> MNYNLSKYPDDVSRLFKPRPPLSYKRPTDYPYAKRQTNPNITGVANLLSTSLKHYMEEFPEGSPNNHLQRYEDIKLSKIKNAQLLDRRLQNWNPNVDPHIKDTDPYRTIFIGRLPYDLDEIELQKYFVKFGEIEKIRIVKDKITQKSKGYAFIVFKDPISSKMAFKEIGVHRGIQIKDRICIVDIERGRTVKYFKPRRLGGGLGGRGYSNRDSRLPGRFASASTSNPAERNYAPRLPRRETSSSAYSADRYGSSTLDARYRGNRPLLSAATPTAAVTSVYKSRNSRTRESQPAPKEAPDY;> MPKFYCDYCDTYLTHDSPSVRKTHCSGRKHKENVKDYYRNKARDIINKHNHKRRHIGKRGRKERENSSQNETLKVTCLSNKEKRHIMHVKKMNQKELAQTSIDTLKLLYDGSPGYSKVFVDANRFDIGDLVKASKLPQRANEKSAHHSFKQTSRSRDETCESNPFPRLNNPKKLEPPKILSQWSNTIPKTSIFYSVDILQTTIKESKKRMHSDGIRKPSSANGYKRRRYGN;> MSALYFQNLPSRPANKENYTRLLLKHINPNNKYAINPSLPLPHNKLQISSQPLMLLDDQMGLLEVSISRSSKMTNQAFLTFVTQEEADRFLEKYTTTALKVQGRKVRMGKARTNSLLGLSIEMQKKKGNDETYNLDIKKVLKARKLKRKLRSDDICAKKFRLKRQIRRLKHKLRSRKVEEAEIDRIVKEFETRRLENMKSQQENLKQSQKPLKRAKVSNTMENPPNKVLLIQNLPSGTTEQLLSQILGNEALVEIRLVSVRNLAFVEYETVADATKIKNQLGSTYKLQNNDVTIGFAKGRRIPGLINPWKRRWKKNFIAVSAANRFKKISSSGALDYDIPTTASENLYFQ;> MDKYTALIHDENFSTLTLNVSRYPKSLAYWEKLLNYIVKASAPICKSTEPQLLKLIRCTYSSMLNEFPYLENYYIDFALLEYKLGNVSMSHKIFQRGLQAFNQRSLLLWTSYLKFCNNVISHQKQLFKKYETAEEYVGLHFFSGEFWDLYLEQISSRCTSSKKYWNVLRKILEIPLHSFSKFYALWLQRIDDIMDLKQLSQLTSKDELLKKLKIDINYSGRKGPYLQDAKKKLKKITKEMYMVVQYQVLEIYSIFESKIYINYYTSPETLVSSDEIETWIKYLDYTITLQTDSLTHLNFQRALLPLAHYDLVWIKYSKWLINSKNDLLGAKNVLLMGLKFSLKKTEIIKLLYSVICKLNEYVLLRNLLEKIESSYSDNVENVDDFEIFWDYLQFKTFCQNSLYSSRYSDSQSNGLLNKELFDKVWKRLSCKEKKSGQEILLNNLVQFYSKDTVEFVEKNIFQKIIEFGWEYYLQNGMFWNCYCRLIYFDTSRSYLDKRQYIVRKIWPQIDKKFAQSVLPSLTEFCESYFPEEMDTLEEMFTEEP;> MPDETNFTIEDIEPRPDALRGLDTQFLQDNTALVQAYRGLDWSDISSLTQMVDVIEQTVVKYGNPNDSIKLALETILWQILRKYPLLFGFWKRFATIEYQLFGLKKSIAVLATSVKWFPTSLELWCDYLNVLCVNNPNETDFIRNNFEIAKDLIGKQFLSHPFWDKFIEFEVGQKNWHNVQRIYEYIIEVPLHQYARFFTSYKKFLNEKNLKTTRNIDIVLRKTQTTVNEIWQFESKIKQPFFNLGQVLNDDLENWSRYLKFVTDPSKSLDKEFVMSVFDRCLIPCLYHENTWMMYIKWLTKKNISDEVVVDIYQKANTFLPLDFKTLRYDFLRFLKRKYRSNNTLFNNIFNETVSRYLKIWPNDILLMTEYLCMLKRHSFKNSLDQSPKEILEKQTSFTKILETSITNYINNQIDAKVHLQTLINDKNLSIVVVELIKTTWLVLKNNMQTRKYFNLYQKNILIKNSVPFWLTYYKFEKSNVNFTKLNKFIRELGVEIYLPTTVMNDILTDYKTFYLTHSNIVTYESSIIDSNTFDPILYPELKMSNPKYDPVLNTTANVDWHKKTEWKEAGHIGITTERPQISNSIIECNSGTLIQKPISLPNFRNLEKINQVKINDLYTEEFLKEGK;> MSYKQTTYYPSRGNLVRNDSSPYTNTISSETNNSSTSVLSLQGASNVSLGTTGNQLYMGDLDPTWDKNTVRQIWASLGEANINVRMMWNNTLNNGSRSSMGPKNNQGYCFVDFPSSTHAANALLKNGMLIPNFPNKKLKLNWATSSYSNSNNSLNNVKSGNNCSIFVGDLAPNVTESQLFELFINRYASTSHAKIVHDQVTGMSKGYGFVKFTNSDEQQLALSEMQGVFLNGRAIKVGPTSGQQQHVSGNNDYNRSSSSLNNENVDSRFLSKGQSFLSNGNNNMGFKRNHMSQFIYPVQQQPSLNHFTDPNNTTV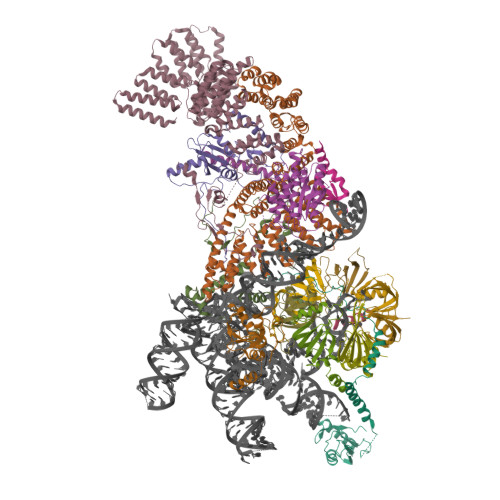FIGGLSSLVTEDELRAYFQPFGTIVYVKIPVGKCCGFVQYVDRLSAEAAIAGMQGFPIANSRVRLSWGRSAKQTALLQQAMLSNSLQVQQQQPGLQQPNYGYIPSSTCEAPVLPDNNVSSTMLPGCQILNYSNPYANANGLGSNNFSFYSNNNATNTQATSLLADTSSMDLSGTGGQQVIMQGSEAVVNSTNAMLNRLEQGSNGFMFA;> MRPRRRGLAYHHTKPKGQLSQGHYPTTSNDGQRRKVGNSEAFQSFDIWKNLDRIRSTKKNAGQFIKGSLLILPMRTEDKQQFDECMDELHKYISKDILRCYPQKEQKDEGMLFYIVLKDFNILDSCFVLSVLLAFQKRLWMAPSEKSYFRVPKNINLTGSFYLPKNIETGRGHIITSYRREQPSSSIVEVGFNVVPDFQQFQVKACHVSKFMNELSNFFSQVEFGKCEANVINYFKREYNRTYSQISLALYELPLIGDGLFDIKSYISKTRPIIETSKAQMIKHISEMKAYNEISGLQGDQFPRQQRPLSNSPSSNSISSSQTIEAGATSYQTQPQRHAVNKPSNVLNSSNRHSGPKTFEDGRYSEGNKPGFMTQDEIKQHCIGTIKASMDAVKKKSSYQILKTYVRCPRQNYIDIVYQNLNDLRSKTNCNIVVLNLNNLHESQMWLESLNTTNYTIFAQAPHPSTIRVISIGGVGEYIVKALELILNILEH;> MRDIVFVSPQLYLSSQEGWKSDSAKSGFIPILKNDLQRFQDSLKHIVDARNS;> MSTMSTPAAEQRKLVEQLMGRDFSFRHNRYSHQKRDLGLHDPKICKSYLVGECPYDLFQGTKQSLGKCPQMHLTKHKIQYEREVKQGKTFPEFEREYLAILSRFVNECNGQISVALQNLKHTAEERMKIQQVTEELDVLDVRIGLMGQEIDSLIRADEVSMGMLQSVKLQELISKRKEVAKRVRNITENVGQSAQQKLQVCEVCGAYLSRLDTDRRLADHFLGKIHLGYVKMREDYDRLMKNNRTTNASKTATTLPGRRFV;> MSKIQVAHSSRLANLIDYKLRVLTQDGRVYIGQLMAFDKHMNLVLNECIEERVPKTQLDKLRPRKDSKDGTTLNIKVEKRVLGLTILRGEQILSTVVEDKPLLSKKERLVRDKKEKKQAQKQTKLRKEKEKKPGKIAKPNTANAKHTSSNSREIAQPSSSRYNGGNDNIGANRSRFNNEAPPQTRKFQPPPGFKRK;> MKLVNFLKKLRNEQVTIELKNGTTVWGTLQSVSPQMNAILTDVKLTLPQPRLNKLNSNGIAMASLYLTGGQQPTASDNIASLQYINIRGNTIRQIILPDSLNLDSLLVDQKQLNSLRRSGQIANDPSKKRRRDFGAPANKRPRRGL;> MSSQIIDRPKHELSRAELEELEEFEFKHGPMSLINDAMVTRTPVIISLRNNHKIIARVKAFDRHCNMVLENVKELWTEKKGKNVINRERFISKLFLRGDSVIVVLKTPVE;> MTMNGIPVKLLNEAQGHIVSLELTTGATYRGKLVESEDSMNVQLRDVIATEPQGAVTHMDQIFVRGSQIKFIVVPDLLKNAPLFKKNSSRPMPPIRGPKRR;> MSNKVKTKAMVPPINCIFNFLQQQTPVTIWLFEQIGIRIKGKIVGFDEFMNVVIDEAVEIPVNSADGKEDVEKGTPLGKILLKGDNITLITSAD;> MSESSDISAMQPVNPKPFLKGLVNHRVGVKLKFNSTEYRGTLVSTDNYFNLQLNEAEEFVAGVSHGTLGEIFIRCNNVLYIRELPN;> MVSTPELKKYMDKKILLNINGSRKVAGILRGYDIFLNVVLDDAMEINGEDPANNHQLGLQTVIRGNSIISLEALDAI Bacterial caseinolytic protease P subunit (ClpP) is important and vital for cell survival and infectivity. The caseinolytic protease P (ClpP) subunit is a compartmentalized structure with two stacked heptameric rings that form a central chamber containing 14 identical catalytic sites sequestered by two protective axial pores. In any case, even the degradation of small oligopeptides depends on some structural factors, and the most important one is the orientation and positioning of the catalytic triads formed by Ser98, His123, and Asp17224. The protein’s mode of action corresponds to that of a chymotrypsin-like protease, and it is described in two main steps: acylation and deacylation.

Aiming to explore and explain this paradoxical effect, we solved and refined the crystal structure of native ClpP from Staphylococcus epidermidis (Se), an opportunistic pathogen involved in nosocomial infections, as well as ClpP in complex with ixazomib at 1.90 Å and 2.33 Å resolution, respectively. The superimposition of both tetradecameric structures displays that the complex is slightly more extended than the apo SeClpP, and the Cα RMSD is 1.63 Å for 1451 atoms. Ixazomib, for example, is a compound that does not affect the integrity of the barrel-like structure, as also observed in ClpPs bound to peptides or other peptidomimetic compounds. Despite the similarity between the overall structures and the high homology between amino acid sequences of ClpPs from different species, a closer look into the monomers exhibits a difference in the Gly-rich region. The structure in this region seems to be more ordered when ixazomib is present. As already stated, the boron atom of ixazomib is covalently bound to Ser98, while the peptide-like portion of the ligand is stabilized by forming hydrogen bonds with amino acids in the active site of ClpP, which cause to some extent cooperative structural arrangements. A comparative analysis with the native SeClpP, the SeClpP-ixazomib complex, and SaClpP Y63A29 structures revealed that the Asn42 side chain in the complex, as well as in the mutant, is shifted to the “down” position (the hydroxyl group is approx. 5 Å distant from Tyr21). It indicates that the boronate compound can control the conformation of the axial pores, even if not bound to the hydrophobic pockets. Based on the previous discussion, here we show an allosteric activation caused by the inhibitor ixazomib. This ligand, at high concentrations, controls allosterically the N-terminal loops in the pores, in a way that globular proteins can be degraded inside the inner chamber of ClpP.

>MNLIPTVIETTNRGERAYDIYSRLLKDRIIMLGSQIDDNVANSIVSQLLFLQAQDSEKDIYLYINSPGGSVTAGFAIYDTIQHIKPDVQTICIGMAASMGSFLLAAGAKGKRFALPNAEVMIHQPLGGAQGQATEIEIAANHILKTREKLNRILSERTGQSIEKIQQDTDRDNFLTAAEAKEYGLIDEVMEPEKHHHHHH[14x]> IDFVYRVDPNPPDVIFRDGFSLLGYNRDLQQLISGRSCAGGSSDSRYIVTTSDINKTYAIARAYYSHSKFKGNLYRYKIRADNNFYSLTPSVNYLESQGGHFNAYEKSMIRLQSEYVSTLS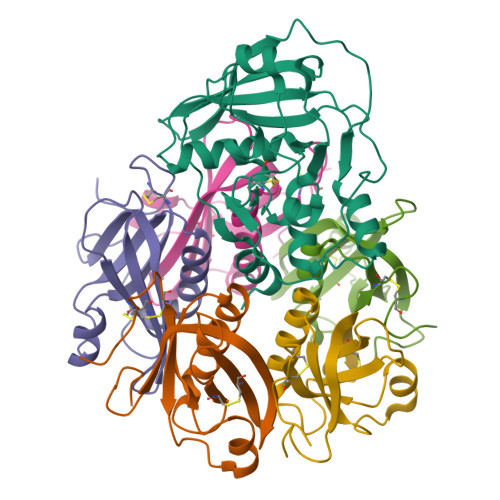ILPENIQKAVALVYDSSTGQIKDGTSTINTDYVSISSVSNPGVIPFLPEPQANTQQRIDAFGSLISSCFSIYSVCQTHRGQKTEVYKMPFYDARPVIQFIISGN;>[3x]EWTGDYENIGYFSHEVISEFHVGQIDGGAYFCIKAVKADGSRSTPLIACSVSNESVWAPSFKVLLEQARYFYVTEQSVRIYYDHNVWTNQPFVNTFSTNALVGLSSCSAATDCFGPGKP;>EWTGDSSINYYSDEVISDFHVGQFNRSAYFCIKTVKKSGEGTPIIACALSHDSKWIPSFNIMLEQARNFYITGHSIRVYVQPNVWSNKSFIEALSSNALVGLSSCSTSECFGPVK[2x]>GASGDVCQDCIQMVTDIQTAVRTNSTFVQALVEHVKEECDRLGPGMADICKNYISQYSEIAIQMMMHMQP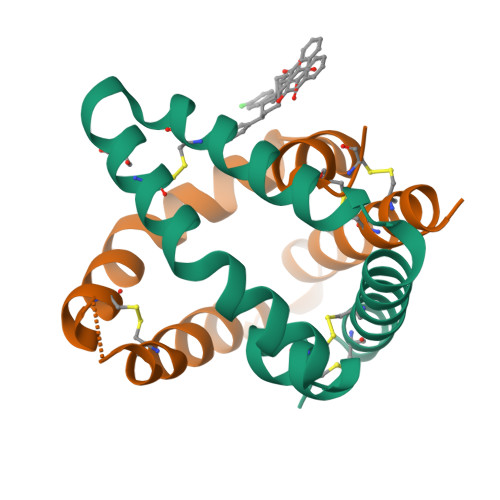KEICALVGFCD[3x]>MGSSHHHHHHSSGLVPRGSHMSEQETRGANEAIDFNDELRNRREKLAALRQQGVAFPNDFRRDHTSDQLHEEFDAKDNQELESLNIEVSVA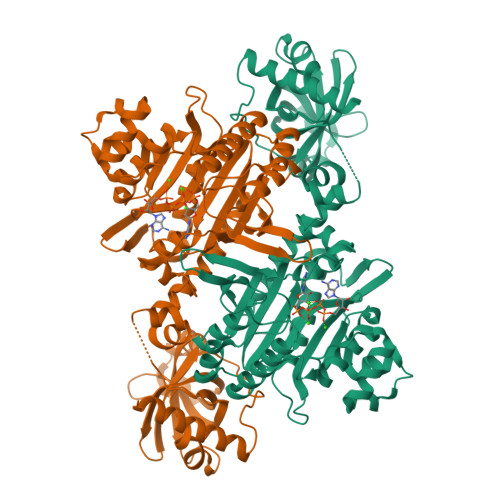GRMMTRRIMGKASFVTLQDVGGRIQLYVARDSLPEGVYNDQFKKWDLGDIIGARGTLFKTQTGELSIHCTELRLLDKALRPLPDKFHGLQDQEVRYRQRYLDLIANDKSRQTFVVRSKILAAIRQFMVARGFMEVETPMMQVIPGGASARPFITHHNALDLDMYLRIAPELYLKRLVVGGFERVFEINRNFRNEGISVRHNPEFTMMELYMAYADYHDLIELTESLFRTLAQEVLGTTKVTYGEHVFDFGKPFEKLTMREAIKKYRPETDMADLDNFDAAKALAESIGITVEKSWGLGRIVTEIFDEVAEAHLIQPTFITEYPAEVSPLARRNDVNPEITDRFEFFIGGREIGNGFSELNDAEDQAERFQEQVNAKAAGDDEAMFYDEDYVTALEYGLPPTAGLGIGIDRMIMLFTNSHTIRDVILFPAMRPQK[3x]> M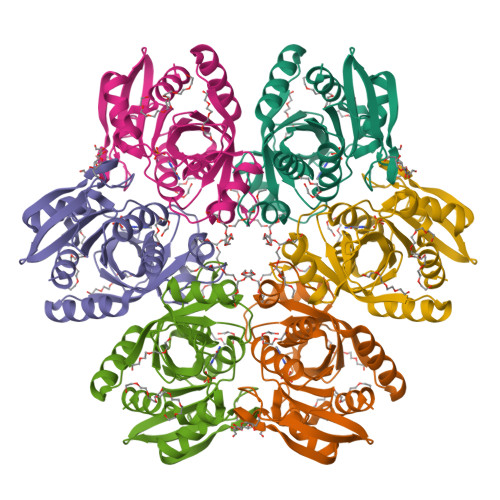TPHINAKIGDFYPQCLLCGDPLRVSYIAKKFLQDAKEITNVRNMLGFSGKYKGKGISLMGHGMGIASCTIYVTELIKTYQVKELLRIGTCGAISPKVGLKDIIMATGASTDSKTNRVRFLNHDLSATPDFELSLRAYQTAKRLGIDLKIGNVFSSDFFYSFETHAFDLMAQYNHLAIEMEAAGLYATAMELNAKALCLCSVSDHLITKEALSPKERIESFDNMIILALEMMS> GPGMDPNTVSSFQVDCFLWHVRKRVADQELGDAPFLDRLRADQASLRGRGSTLGLDIETATRAGKQIVERILKEESDEALKMTMASVPASRYLTDMTLEEMSREWSMLIPKQKVAGPLCIRMDQAIMDKNIILKANFSVIFDRLETLILLRAFTEEGAIVGEISPLPSLPGHTAEDVKNAVGVLI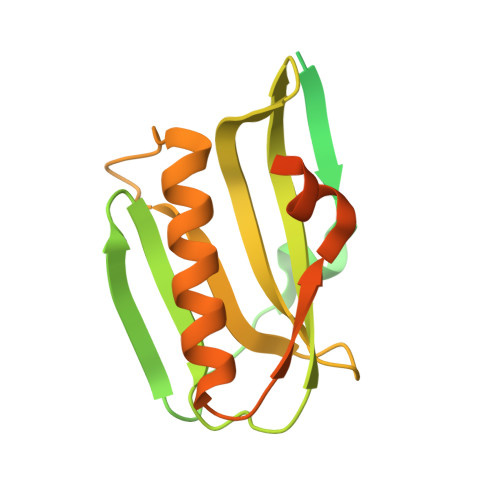GGLEANDNTVRVSETLQRFAWRSSNENGRPPLTPKQKREMAGTIRSEV5-CHLORO-8-METHYL-7-(3-METHYL-BUT-2-ENYL)-6,7,8,9-TETRAHYDRO-2H-2,7,9A-TRIAZA-BENZO[CD]AZULENE-1-THIONE 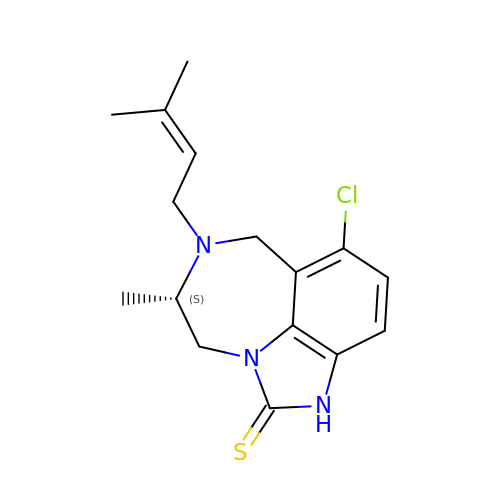| C16 H20 Cl N3 S | ZNFFMCYSMBXZQU-NSHDSACASA-N>[2x]MSNEVEQKKNIKTINDLPGISQTVINKLIEAGYSSLETLAVASPQDLSVAAGIPLSTAQKIIKEARDALDIRFKTALEVKKERMNVKKISTGSQALDGLLAGGIETRTMTEFFGEFGSGKTQLCHQLSVNVQLPPEKGGLSGKAVYIDTEGTFRWERIENMAKALGLDIDNVMNNIYYIRAINTDHQIAIVDDLQELVSKDPSIKLIVVDSVTSHFRAEYPGRENLAVRQQKLNKHLHQLTRLAEVYDIAVIITNQVMARPDMFYGDPTVAVGGHTLYHVPGIRIQLKKSRGNRRIARVVDAPHLPEGEVVFALTEEGIRDAEE

Homologous recombination is a ubiquitous mechanism for maintaining genome integrity and also for generating genetic diversity in sexual reproductive organisms. This reaction is catalyzed by RecA family proteins, including bacterial RecA, archaeal RadA, and eukaryal Rad51 and Dmc1. The current model holds that, in the presence of ATP, the recombinases coat a primary single-stranded DNA (ssDNA) to form a nucleoprotein right-handed helical filament, and initiate a search for a secondary homologous stretches of double-stranded DNA (dsNDA). By contrast, archaeal RadA is a better model for eukaryotic recombinases.

Here we report additional three new crystal structures of left-handed helical filaments. First, the basic structural element of these three new helical filaments is a RadA dimer. The other protomers were then assigned as 2ZUB_B, 2ZUC_B and 2ZUD_B, respectively. A unique property of these left-handed helical filaments, as compared to other known structures of RecA family proteins, is that their DNA binding motifs (i.e., L1, L2 and NTD) are all located at the outermost surface of helical filaments. Moreover, the NTDs are separated a long way from L1 and L2 motifs. We found that the locations of the L1 and L2 motifs in the four left-handed helical filaments are relatively conserved, but in contrast, the NTD locations are quite different. The first hinge region, located between the NTD and the PM, is referred to here as “subunit rotational motif 1 (SRM1)”. Subsequent structural and biochemical analysis revealed that SRM1, a hinge region between the NTD and the PM, is not only responsible for structural flexibility of the NTD but also is important for RadA's function in promoting D-loop formation.> GMSGTANSRRKEVLRVPVIDLNRVSDEEQLLPVVRAILLQHDTFLLKNYANKAVLDALLAGLTTKDLPDTSQGFDANFTGTLPLEDDVWLEQYIFDTDPQLRFDRKCRNESLCSIYSRLFKLGLFFAQLCVKSVVSSAELQDCISTSHYATKLTRYFNDNGSTHDGADAGATVLPTGDDFQYLFERDYVTFLPTGVLTIFPCAKAIRYKPSTMATT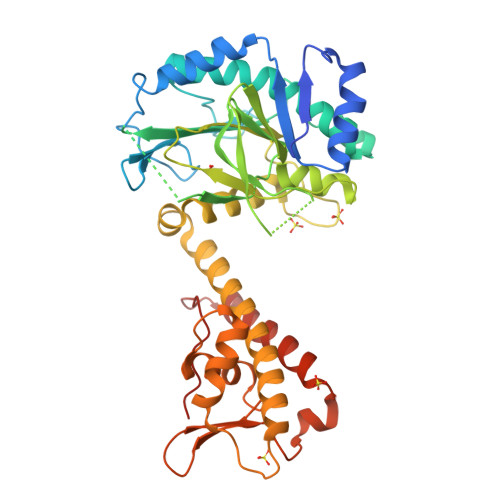DNSWVSIDEPDCLLFHTGTLLARWSQGMHTTSPLQIDPRANIVSLTIWPPLTTPISSKGEGTIANHLLEQQIKAFPKVAQQYYPRELSILRLQDAMKFVKELFTVCETVLSLNALSRSTGVPPELHVLLPQISSMMKRKIVQDDILKLLTIWSDAYVVELNSRGELTMNLPKRDNLTTLTNKSRTLAFVERAESWYQQVIASKDEIMTDVPAFKINKRRSSSN> MRGSHHHHHHTDPNSPLDEENLTQENQDRGTHV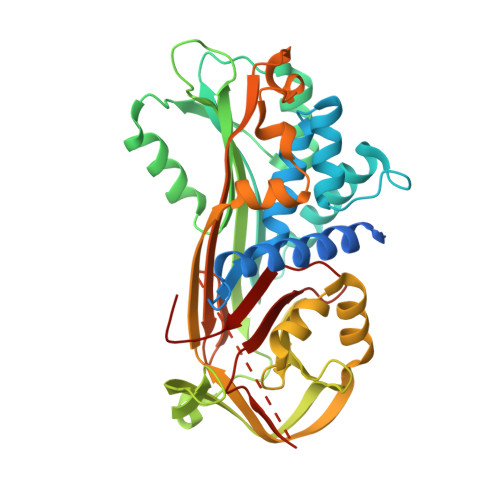DLGLASANVDFAFSLYKQLVLKAPDKNVIFSPLSISTALAFLSLGAHNTTLTEILKGLKFNLTETSEAEIHQSFQHLLRTLNQSSDELQLSMGNAMFVKEQLSLLDRFTEDAKRLYGSEAFATDFQDSAAAKKLINDYVKNGTRGKITDLIKDLDSQTMMVLVNYIFFKAKWEMPFDPQDTHQSRFYLSKKKWVMVPMMSLHHLTIPYFRDEELSCTVVELKYTGNASALFILPDQDKMEEVEAMLLPETLKRWRDSLEFREIGELYLPKFSISRDYNLNDILLQLGIEEAFTSKADLSGITGARNLAVSQVVHKAVLDVFEEGTEASGTTAVKITLLSALVETRTITRFNRPFLMIIVPTDTQNIFFMSKVTNPKQA> GPLGSNPASLYRIDLFITFTDELITFDYKVHGRPVLTFRIPGFGLTPAGRMLVC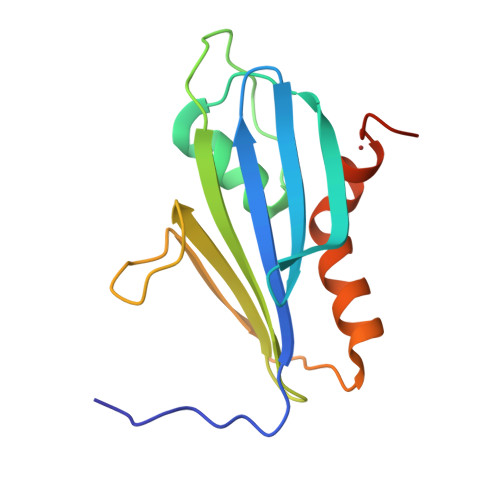MGEKPAHSPFTSSKSLYHVIFTSTCNSFSFTIYKGRYRSWKKPIHDELVDRGYTTFREFFKAVRGYHADYYKQRLIHDVEMNPG>[4x]MKIQGTYTA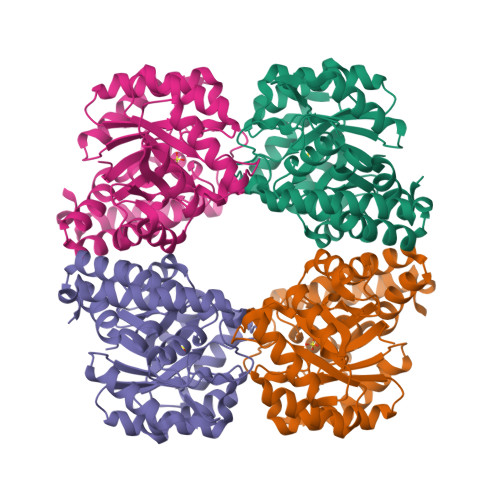IISPFHNGQIDRKALERLLEHQIENRIDGIVPVGTTGESPTLSYEEHIELVRLTAEIVEKRIKIFAGTGSNSTAEAIHLTKEAEKIGVDGVLLVSPYYNRPSQEGLFRHFSAIAASTSLPILLYNIPSRCGVDIAVDTVKRLVEKNKNIVGIKEAGGSVDRVSQLVEALPGEFSILSGDDALTLPFLSVGAVGVVSVASNLFPRPVSALVRLYLEGKPFEARQLHQTLYPLFRDLMIETNPVPVKTALAMEGLTDLELRLPLAPLQPQNLEKLKTTLSRTKEKLAKVEHLWA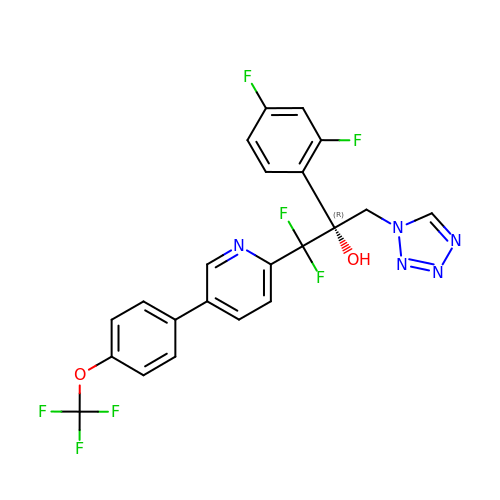(2R)-2-(2,4-difluorophenyl)-1,1-difluoro-3-(1H-tetrazol-1-yl)-1-{5-[4-(trifluoromethoxy)phenyl]pyridin-2-yl}propan-2-ol | C22 H14 F7 N5 O2 | NCEHACHJIXJSPD-FQEVSTJZSA-N> HHHHHHTILGIAATIFIVVGGTLFYRNFIVPKQAAQYYDQGLTLIREAGAYPKNSETRKRKFFEAEESFARGENILPNHLKYLNLYGIEYTRVEEYDRAFEKLFGKVSPDFGAGGEEPSSNAWDKREKVPIITLAKGQVWDNSK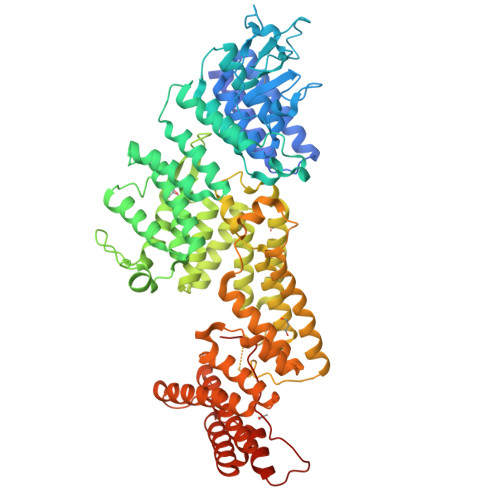LPIAGKVGSENRMTLIAQDGIQRKILKAGAYIVMRLEKQTHDNPTYKNLGRFHSSIMPSFTESSLGGGKYKNDQLAINFYKQVYTDGNEPYDEESTAGIAKIYYNRREFGKAASFYNKIVEIDPSSPMGQGGLLSTYIEMWKEDGNPQFVINHHRQIKNNLEIEKKLSLHVLSKLASFYTNLNKKELRIRYNINPIDQVSGMEVNDNALEILDLIYHKTEKDPITGTEIEGSNYAEGYYQRGRYFASIKESIQARRFFEKAATLDPAHYLASMELGENAIRLANFGEADKLLNESLKRFENFKQSYGAREEDETLIQGNVGRIYFDKARIQYLSAAGIHEKDKITEFPGRKIYPFRARAAMDTVAKTRSMELKNSLEGFSKAESVQTDENEYTLIRRWRTPLPPEIQRELRYFKGWVDYMSGDFAASLNEWSGFEDEEEYNHSTLLMGKANAFFYTGQYKASLGNYLKVQDDMEEKLLNMGLPKPDDPYHQEVYQTLVAAYNNIGAVYEKQGNTSEALKHYWKAIETARKINEVSEIAMSNKDLMFKKEAIGQDPLLEDWLSPTLDSIKKLTRE Pseudouridylation is the most common RNA modification and is observed within tRNA, rRNA, ncRNA and mRNAs. Alternatively, an RNA recognition mechanism that does not rely on guide RNA factors is employed by stand-alone PUS enzymes that independently recognize and modify their targets. More recent data have suggested that PUS1 is the predominant PUS to modify uridines in mRNA. The structures illustrate how PUS1 recognizes and binds a helical RNA duplex and enable the identification of RNA-contacting amino acid residues that make extensive contacts with each RNA strand to orient and guide the RNA into the active site of the enzyme.

To further examine the interactions of bound RNA with a catalytically competent version of the enzyme (in which the catalytic aspartate at position 134 was restored) we altered the RNA ligand by substituting a 5-fluoro-uracil (5-FU) base at position number 1, reasoning that it might be captured in a suicide complex by the enzyme after being flipped into the active site and subsequent nucleophilic attack by the carboxylate of D134. RNAs harboring such substitutions have previously been demonstrated to act as mechanism-based inhibitors of pseudouridine synthase enzymes and have been used to demonstrate the structural mechanism by which the target base gains access to the enzyme’s active site. Although the space group and corresponding lattice packing arrangement of the protein-RNA enzyme complex was completely unrelated to the packing of the C2 space group of the PUS1D134A:RNA complex, the same RNA duplex, and the same position of two independently bound protein subunits was observed. The RNA duplex and second bound protein molecule is again generated by the application of crystallographic two-fold rotation symmetry on the contents of the asymmetric unit (which again corresponds to a single protein subunit and a single RNA chain). Structural superposition of an RNA-bound monomer or dimer from the two crystal structures produced rmsd values of 0.63 Å and 1.47 Å, respectively. Beyond providing an independent confirmation of the binding of two copies of the enzyme to an RNA duplex in a symmetric arrangement, the resulting electron density map, after several initial rounds of rebuilding and refinement, displayed a significant feature of positive difference density in the active site that might be indicative of low occupancy (ultimately estimated at less than 10% in refinement) by the 5’ 5FU nucleobase of the RNA. However, the combination of lower resolution and mixture of density features surrounding that base prevented us from unambiguously modeling the bound RNA in a state corresponding to a trapped catalytic complex.

> MSEENLRPAYDDQVNEDVYKRGAQSKLTKARKADFDDEKDKKKDNDKHIDKRPKSGPRLDENGNPLPKEPRLPKRKVAVMVGYCGTGYHGMQYNPPNPTIESALFKAFVEAGAISKDNSNDLKKNGFMRAARTDKGVHAGGNLISLKMIIEDPDIKQKINEKLPEGIRVWDIERVNKAFDCRKMCSSRWYEYLLPTYSLIGPKPGSILYRDIEESKTELPGVLDEDLESKEFWEEFKKDANEKFSTEEIEAILAYVPPARDEFDINEELYQKVKKYKQLENAHRRRYRISAAKLAKFRASTSQYLGAHNFHNFTLGKDFKEPSAIRFMKDIKVSDPFVIGDAQTEWISIKIHGQSFMLHQIRKMVSMATLITRCGCPVERISQAYGQQKINIPKAPALGLLLEAPVFEGYNKRLEQFGYKAIDFSKYQDEVDKFKMKHIYDKIYKEEVDENVFNAFFSYIDSFNKVTGAQGEETADKSGPAVQKSIFEFLTAKGIPGLTDAPESNKKIKQRKRMEEEEAASKKAEISSTTQSNEPEVQPEAAAN> GSGETGEKTPETVALLQNLKQAERKGILFGHHDDTAYGIGWEGDKGRSDVKSVCGAYPGVMSFDLGEIELGGTHNLDKVSFAHLREYIIEQYARGGMISLSWHVRNPKTGGDSWDVTDSTVVASVMQGGENHVKMLEWIDRVADFLLSLKTKEGVLIPVVFRPWHEHTGSWFWWGKDLCSSEQYKTLWRMTNDRLRLKGVNNVLLAYSPGMESDTVEEYLERYPGDDIIDVLGTDVYQFERSQYIKQLNKMLTILTEAGKKHDKPIALTETGLEGIPDSLWWTGTLLPVIEKYPLSYVLVWRNAREKSTHYYAPYPGQVSADDFVKFSRSPKILFVGDNFELYKLEHHHHHH

A putative β-mannan PUL was previously identified in B. ovatus ATCC 8483 (bacova_02087–02097) and shown to be transcriptionally up-regulated when galactomannan or glucomannan was included in the culture medium. This PUL contains the genes bacova_02092 and bacova_02093, which encode the putative GH26 β-mannanases BoMan26A and BoMan26B, respectively. Clan GH-A enzymes share a (β/α)8-barrel fold, a conserved retaining catalytic mechanism, and essential catalytic residues (nucleophile and acid/base). β-Mannanases generally have an active site cleft with a varied number of sugar-binding subsites (−2, −1, +1, +2, etc.), with the reducing sugar being located in the + subsites and the target mannosidic bond connecting the sugars in subsites −1 and +1. BoMan26A has M2 as a clear main product when hydrolyzing all tested mannan substrates. Galactomanno-oligosaccharides are further processed in the periplasm, degalactosylated by BoGal36A and subsequently hydrolyzed into mannobiose units by the β-mannanase BoMan26A.

A 3D structure of BoMan26A was obtained using molecular replacement with the structure of GH26 mannanase C from Cellvibrio japonicus (CjMan26C), the closest homologue with a solved structure. The protein displays the expected β8α8-barrel structure, which is conserved in all GH26 enzymes, with the active site located in a cleft. The catalytic residues Glu-188 (acid/base) and Glu-292 (nucleophile) are located at the ends of β-strands 4 and 7, respectively, and are conserved within GH26 (40) and other clan GH-A families. Comparing the structure of BoMan26A with that of CjMan26C with G1M4 shows that the −2 to +1 subsites are largely conserved, with residues His-125, His-187, Trp-193, Tyr-259, and Trp-323 being conserved throughout GH26 (28). Beyond subsite +2, the active site cleft becomes more open in BoMan26A, lacking several residues equivalent to those in CjMan26C. Because of crystal packing, the fused His tag of one monomer is situated in the active site cleft of the adjacent monomer, potentially aiding the formation of the crystals. Based on substrate binding in CjMan26C, loop 2 appears to close off the area beyond the −2 subsite in BoMan26A, despite 18O labeling showing that BoMan26A is capable of accommodating a mannosyl in the −3 subsite. The low B-factor of loop 2 indicates low flexibility in the crystal structure; however, a stabilizing factor may be that Asp-99 in loop 2 hydrogen bonds to His-373, the last residue in the His tag of the neighboring molecule in the crystal. Thus, loop displacement to generate a −3 subsite cannot be ruled out in solution, especially because the equivalent loop is shorter in other endo-acting β-mannanases, giving a more open active site cleft. Taken together, the more open +3 subsite and the potential loops 2 and 8 conformational changes allowing a −3 subsite may explain the endo-activity we observed for BoMan26A but was not observed for CjMan26C.> ADTLDNVNLVSSPVHSGFLVSFMVDARGGS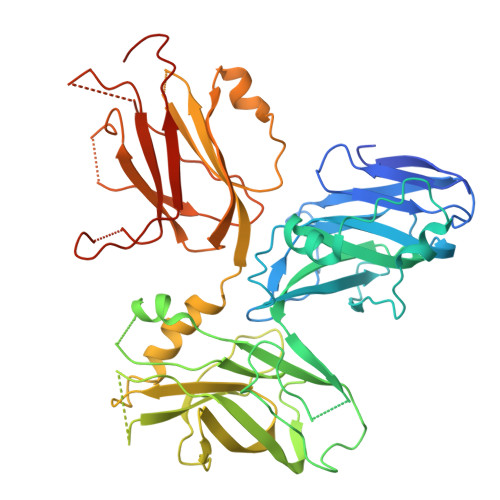MRGSRHHGMRIIIPPRKCTAPTRITCRLVKRHKLANPPPMVEGEGLASRLVEMGPAGAQFLGPVIVEIPHFGSMRGKERELIVLRSENGETWKEHQFDSKNEDLSELLNGMDEELDSPEELGTKRICRIITKDFPQYFAVVSRIKQESNQIGPEGGILSSTTVPLVQASFPEGALTKRIRVGLQAQPVPEETVKKILGNKATFSPIVTVEPRRRKFHKPITMTIPVPPPSGEGVSNGYKGDTTPSLRLLCSITGGTSPAQWEDITGTTPLTFIKDCVSFTTNVSARFWLADCHQVLETVGLASQLYRELICVPYMAKFVVFAKTNDPVESSLRCFCMTDDRVDKTLEQQENFEEVARSKDIEVLEGKPIYVDCYGNLAPLTKGGQQLVFNFYSFKENRLPFSIKVRDTSQEPCGRLSFLKEPKTTKGLPQTAVCNLNITLPAHKKAEKADRRQSFTSLALR>ETGGCTNVDSPNFNFQANMDDDSCDAKVTNFTFGGVYQECTELSGDVLCQNLEQKNLLTGDFSCPPGYSPVHLLSQTHEEGYSRLECKKKCTLKIFCKTVCEDVFRVAKAEFRAYWCVAAGQVPDNSGLLFGGVFTDKTINPMTNAQSCPAGYIPLNLFESLKVCVSLDYELGFKFSVPFGGFFSCIMGNPLVNSDTAKDVRAPSLKKCPGGFSQHLAVISDGCQVSYCVKAGIFTGGSLLPVRLPP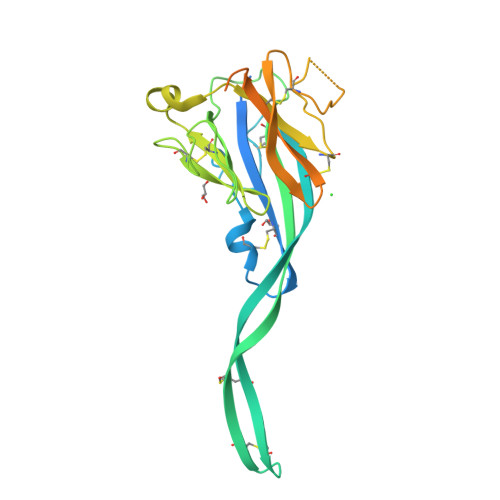YTKPPLMSQVATNTVIVTNSETARSWIKDPQTNQWKLGEGTKHHHHHH[2x]>SIWSRVVQFGTGWGFWVSGHVFITAKHVAPPKGTEIFGRKPGDFTVTSSGDFLKYYFTSAVRPDIPAMVLENGCQEGVVASVLVKRASGEMLALAVRMGSQAAIKIGSAVVHGQTGMLLTGSNAKAQDLGTIPGDAGCPYVYKKGNTWVVIGVHVAATRSGNTVIAATHGEPTLEAWQA[2x]

Whereas ORF2, ORF3 and ORF4 each encode single proteins, ORF1 codes for a large polyprotein (∼190 kDa) that is processed by the virally-encoded protease at five specific sites to release the six ‘mature’ non-structural proteins (NS1/2–NS7)—and an array of functional precursors—that are required for virus replication. The viral NS6 protease present within the C-terminal half of the polyprotein performs all the processing, including its own autocatalytic release from the precursor (Liu, Clarke & Lambden, 1996; Belliot et al., 2003; Sosnovtsev et al., 2006; Scheffler et al., 2007). Norovirus NS6 is a cysteine protease with a chymotrypsin-like fold: two β-barrel domains separated by a cleft that contains a Cys-His-Asp/Glu catalytic triad similar in arrangement to the Ser-His-Asp triad characteristic of serine proteases. To this end we extended an inactive MNV NS6 construct (which incorporates a C139A mutation to knock out the active site nucleophile) by adding residues from NS7, which is immediately downstream in the polyprotein.

To investigate the structural variation in substrate recognition we also made an NS6 chimera which interchanged the residues P4-P4′ of the NS6-7 cleavage junction with the sequence of the NS2-3 junction from MNV (NS6 4′ 2|3). NS6 4′ 2|3 crystallised with two molecules in a P1 unit cell. The modelled monomers start at residue 4 and end at residue 182; in contrast to the other structures reported here, the A chain lack density for the tip of the eII-fII loop so residues 162–163 were omitted. The A and B chains each extend their C-termini into the cleft formed between the bII-cII and eII-fII loops of a neighbouring molecule. The packing arrangements are distinct but rather similar and, once again, lack specific contacts that are consistent with productive substrate binding.> GAGTLIKDNLKRDLITSLPFEISL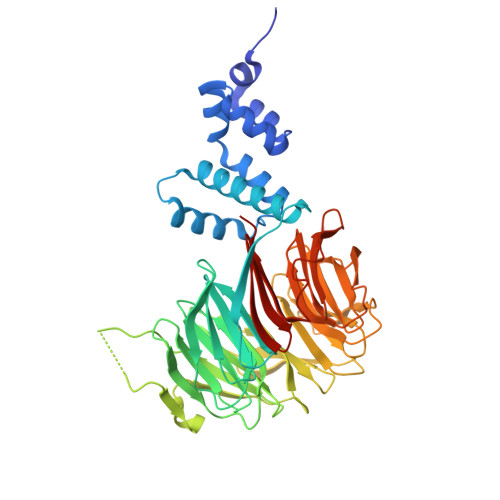KIFNYLQFEDIINSLGVSQNWNKIIRKSTSLWKKLLISENFVSPKGFNSLNLKLSQKYPKLSQQDRLRLSFLENIFILKNWYNPKFVPQRTTLRGHMTSVITCLQFEDNYVITGADDKMIRVYDSINKKFLLQLSGHDGGVWALKYAHGGILVSGSTDRTVRVWDIKKGCCTHVFEGHNSTVRCLDIVEYKNIKYIVTGSRDNTLHVWKLPKESSVPDHGEEHDYPLVFHTPEENPYFVGVLRGHMASVRTVSGHGNIVVSGSYDNTLIVWDVAQMKCLYILSGHTDRIYSTIYDHERKRCISASMDTTIRIWDLENGELMYTLQGHTALVGLLRLSDKFLVSAAADGSIRGWDANDYSRKFSYHHTNLSAITTFYVSDNILVSGSENQFNIYNLRSGKLVHANILKDADQIWSVNFKGKTLVAAVEKDGQSFLEILDFS>MMTEKDEGKRLQLSLDKLGDWEKEMSQVEREAEIYRIKKTQPMYAKRRSILKEIPKFWYIVLAENDDFADYISPDDLKYLEYIDDIYVYYPIVDDEAGHFKDFNITVTFGKNPYIPEQEITKKFKIVIQEDGDERIVSESVEVKWPHELSKINPSVIKEKYKGKDKKDMSAKDKKNYRLGMKSFFSWFNWTGEKPGKEFRNGEDLATLLSEDLYLNALKYYII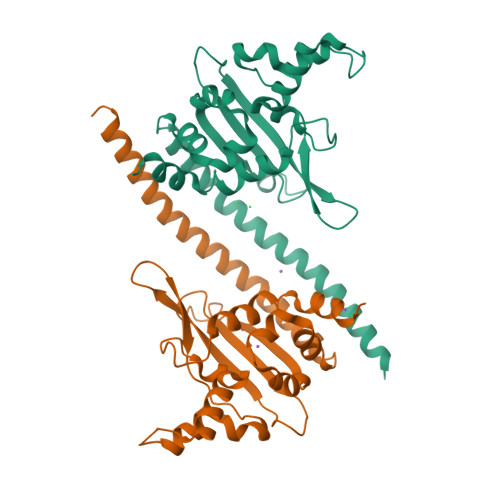ALSPLEHHHHHH[8x]2-chloranyl-1,3-thiazole-5-carboxylic acid | C4 H2 Cl N O2 S | 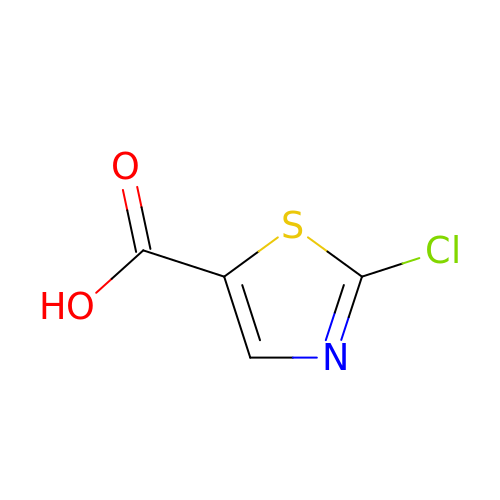HNJOKQPEJIWTRF-UHFFFAOYSA-N6-chloro-N-pyrimidin-5-yl-3-{[3-(trifluoromethyl)phenyl]amino}-1,2-benzisoxazole-7-carboxamide | C19 H11 Cl F3 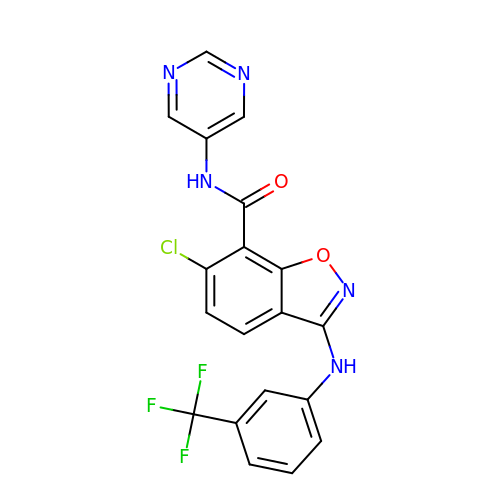N5 O2 | FEGRQUWSKADGSP-UHFFFAOYSA-N> MRGSHHHHHHGSGLKWTDSREIG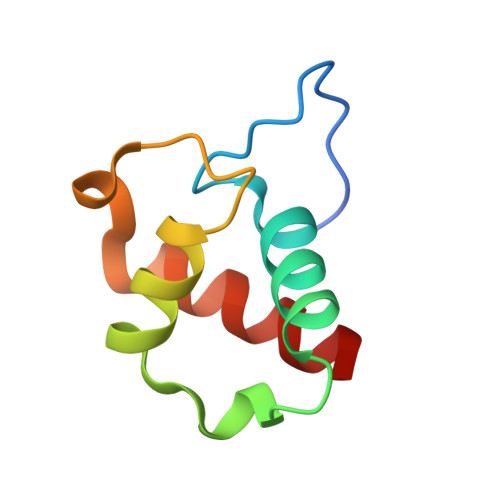EALYDAYPDLDPKTVRFTDMHQWICDLEDFDDDPQASNEKILEAILLVWLDEAE>[2x]GPGSMTQTVKDLAAAIRSGDRAALPRAITLVESTRADHRERAQELLLELMPDAGRAMHVGITGVPGVGKSTSIEALGMHLIEQ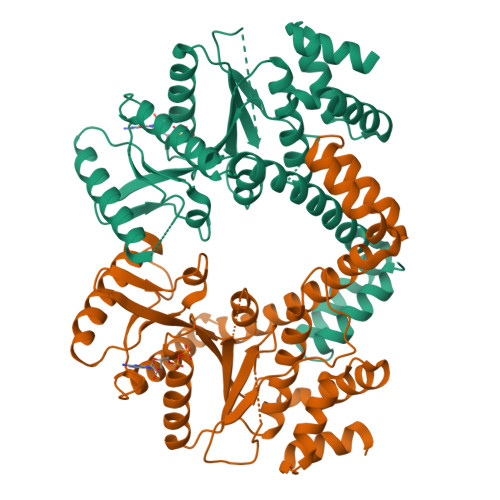GHRVAVLAVDPSSVRSGGSILGDKTRMARLAVHPDAYVRPSPSSGTLGGVAKATRETIVLLEAAGFDVVLVETVGVGQSEVTVADMVDTFVFLTLARTGDQLQGIKKGVLELADIVVVNKADGEHAVEARKAARELAGAMRLIYPRETLWRPPVLTMSALEGTGVAELWETVLKHRQVLIDAGEFEKRRRDQEVNWMWTMVRDAVIDRVMTSPGVREIRAEVERQVREGELTAALAAQRLLDAAELR>[5x]MHNLQQLLPTRSLIWIFSFLTSISIWCTVAHAETEGRVQHFTGYIEDGRGIFYSLPDMKQGDIIYASMQNTGGNLDPLVGIMAEEIDPAVSLGQVLEKALASENDLISELTAVADRIFLGWDDDGGKGYSASLEFTIPRDGTYHIFAGSTITNQRLDKFQPTYTTGSFQLILGLNAPQVISGEGEPEGEVFASLASLEIKPEAHVQELEIRLDKDTRYLTQHTRNLQPGDTFHALVEPIGEAPLPRLRLTDSGGKPLAFGLIDQPGESVELNYTCDQDICELVVHVDGTDGQKDSGEAVYRLLVGINAPNLRESGQTPVGSSVFLESDLVTVGLAVDQIVGVDQRSENFSVVGTLKLSWHDPKLGFSPDQCGCTVKSFEDASIRAVAGEINLPLPSFSFYNQQGNRWSQNQVIFVTPDGRASYFERFTVTLQAPDFDFLAYPFDRQKFSIKVDLAVPTNMFIFNEIERFQQVVGDQLGEEEWVVTSYSQEITEVPFERGSTNSRFTTTLLVKRNLEYYILRIFVPLFLIISVSWVIFFLKDYGRQLEVASGNLLVFVAFNFTISGDLPRLGYLTVLDRFMIVSFCLTAIVVLISVCQKRLGAVGKQAVAAQIDTWVLVIYPLVYSLYIIWVYLRFFTDHIGW

Pentameric ligand-gated ion channels (pLGICs) constitute a family of receptors responsible for the rapid conversion of chemical to electrical signals in most kingdoms of life. To date, the only pLGIC in which an NTD has been partially characterized is DeCLIC, derived from a symbiotic sulfate-reducing deltaproteobacterium related to Desulfofustis glycolicus. The DeCLIC NTD accounts for roughly half the total receptor mass, and appears to accelerate activation and deactivation of the channel. Like several pLGICs, DeCLIC has been shown to be inhibited by calcium ions (Ca2+), mediated at least in part by a calcium-binding site at the ECD-TMD interface.

We then collected data in the absence of calcium, ensured by adding 10 mM ethylenediaminetetraacetic acid (EDTA) to the nanodisc-reconstituted sample. In order to identify potentially asymmetric conformations, we initially processed the resulting dataset without imposing symmetry, and identified two classes. In a second class (asym, 2.7 Å, 42 % of assigned particles), one NTD1 lobe was even more poorly resolved than the others, only clearly visible in a low-pass filtered map. Still, application of 3DFlex and DeepEMhancer enabled building of 80 % of NTD residues. Under calcium-chelating conditions, an additional class could be reconstructed in which one set of adjacent NTD1 and NTD2 lobes was even more poorly resolved and displaced from the symmetric pentamer, consistent with a heterogeneous asymmetric ensemble in the absence of calcium. The asym calcium-free conformation further differed from the calcium-containing structure at one NTD1 and adjacent NTD2 lobes. The asymmetric NTD2 lobe was associated with relatively poor density, but could be built in an alternative pose, displaced upward (away from the membrane plane) and rotated counter-clockwise (viewed from the periplasm) relative to the sym-like arrangement. The NTD1 lobe complementary to this asymmetric NTD2 exhibited even lower local resolution; although its poor definition precluded model building, low-pass filtering indicated a pose displaced outward from the central axis. Interestingly, a similar translocation was predicted by previous MD simulations and small-angle scattering measurements. Thus, depletion of calcium from the NTD2(+)/NTD1(−) interface enabled their partial mobilization and displacement in a subset of particles.>SKKRQWALEDFEIGRPLGKGKFGNVYLAREKQSKFILALKVLFKAQLEKAGVEHQLRREVEIQSHLRHPNILRLYGYFHDATRVYLI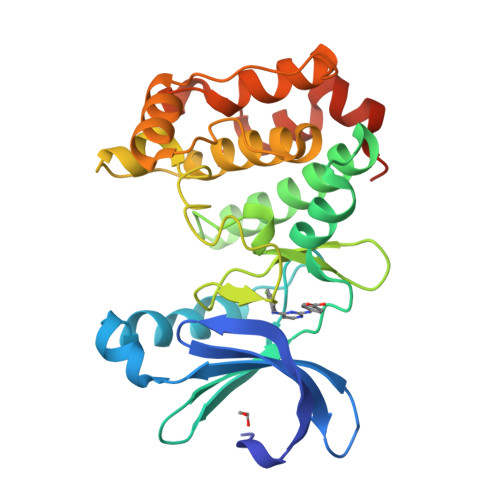LEYAPLGTVYRELQKLSKFDEQRTATYITELANALSYCHSKRVIHRDIKPENLLLGSAGELKIADFGWSVHAPSSRRDTLCGTLDYLPPEMIEGRMHDEKVDLWSLGVLCYEFLVGKPPFEANTYQETYKRISRVEFTFPDFVTEGARDLISRLLKHNPSQRPMLREVLEHPWITANSSKPSNCQNKESASK[2x]(S)-1-(2-AMINO-2-CARBOXYETHYL)-3(2-CARBOXYTHIOPHENE-3-YL-METHYL)-5-METHYLPYRIMIDINE-2,4-DIONE | C14 H15 N3 O6 S | 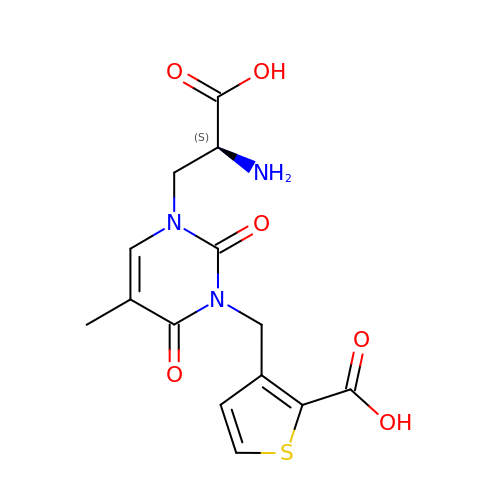ZTAZUCRXCRXNSU-VIFPVBQESA-N> LQQERTKLRPVAMVRPTVR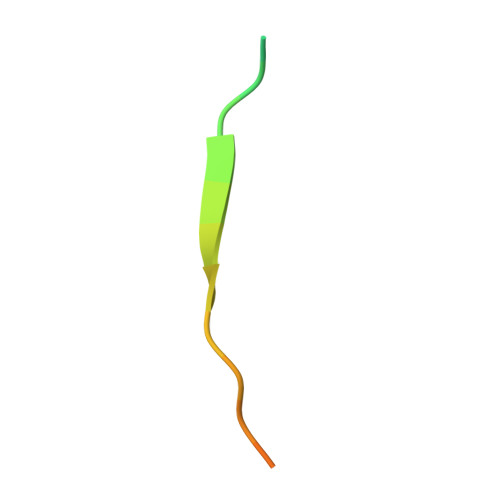VQPQL>ADLSPEEQIETRQAGYAFMAWNMGKIKANLEGEYNADQVRAAANVVA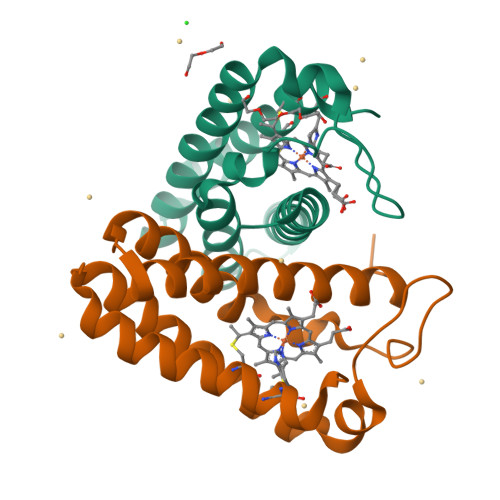AIANSGMGALYGPGTDKNVGAVKTRAKPELFQNLEDVGKLARDLGTAANALAAAAATGEANAVKSAFADVGAACKACHQKYRAD[2x]> SMGKTLRFEIVSGVNKGYF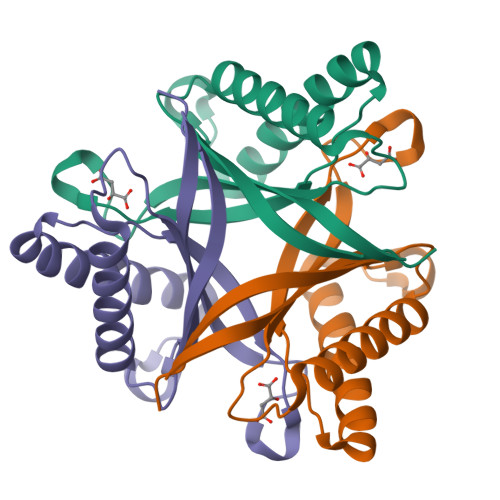HTNSQSESLDLVGGIWQKIAKEEFEKSNIYVSAVIKPSKTVYNQEWGCPENGEETVVLTGVANEEFVDDIEKWKDTVIKLAKELKNQMKQSTLTCEFIETELHYFK>MKISIIGTGRVGSSTAFALINAAVADEIVLYDLNKEMAEGEALDLLHATTFHKRMIIRAGEYSDIEGSDIVLITAGAAQKPGETRLDLTIKNAKIIKGISENIKKYAPNTLIINITNPVDVMSYVVWKVTGFESNRVIGTGTILDTARLRALIGKNCGVSPMSVHAYIIGEHGDSELAAWSSAMIGGVPIKGFCRNCPYKDNCNKDLSKIFDDVKNSAYTIISKKGATNYGIASATTALVESIIKNEGRVYTPSVLLDDVYIGYPAVIN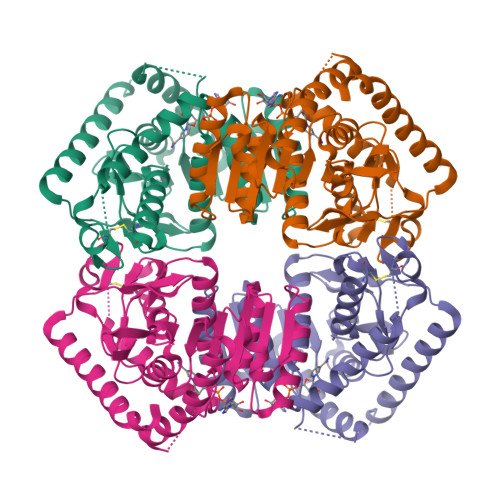KDGVERTIDITLNDEETEKFESSKSIIKEYLESIKNLL[2x]> MSLPLLRPFETVSLENAVEDLVVRFILNVPPEDLSTVERVLFHFEEASWFYTDFVKLMNPYLPNLSIKSFSKIVIDICPLIWNWDITPENALVKFSNYKKTIPVRGAAIFNDSLSKILLLRGINSKHWSFPRGKIGKDEDDVACCIREVKEQTGFDLTGFIDADQYVERNMNGKNFKIFLVKGVPEDFEFKPEHKNEIQAIEWKDFKKLSKAITKNEGSAKVFLVNSMIRP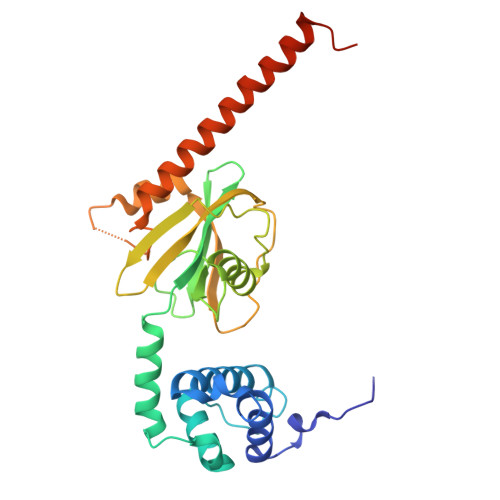LSLYVKNEKRAKDENKLKLYAEEHLKSILGLNKKENKIVLDAGR> DFSTIPIDYVKAKDPNTIDFCLSYLELYHTTKAVKACTPFSFILGSDAGMQRATETTESLYWGKVILDINPNLSPLVNTTIVLEIESMLSSNSINRSENKRITRYIEKENFVNESSERFEFFKSMELSHLSTAYDVYVTFIGFKIDL

In this study, we report a detailed characterization of ΦCjT23, an icosahedral temperate ssDNA phage with an inner lipid membrane, isolated earlier from a strain of Flavobacterium (previously Cytophaga). The virion structure determined by cryogenic electron microscopy reveals similarities to members of the viral kingdom Bamfordvirae that currently consists solely of dsDNA viruses with a major capsid protein composed of two upright β-sandwiches. The minimalistic structure of ΦCjT23 suggests that this phage serves as a model for the last common ancestor between ssDNA and dsDNA viruses in the Bamfordvirae. Both ΦCjT23 and the related phage FLiP infect Flavobacterium species found in several environments, suggesting that these types of viruses have a global distribution and a shared evolutionary origin.

Earlier, we reported a phylogenetic connection between phage PM2 and the ssDNA phage FLiP (Finnlakevirus FLiP, Finnlakeviridae), which infects flavobacteria. Structurally, however, the two share the same capsid organization, characterized by the triangulation (T) number pseudo T = 21 dextro. Following the approach applied to the MCPs, we calculated a localized reconstruction of the internal part of ΦCjT23 spike (penton domain), in addition to the FLiP penton base from our previously published data. The resolutions of the localized reconstructions for ΦCjT23 and FLiP were 3.4 and 4.0 Å, respectively. This was sufficient to build the corresponding atomic models de novo. As expected, the structure of the FLiP penton revealed a pentamer formed by five copies of protein P12 (encoded by orf12) with the canonical β-sandwich fold, similar to penton base proteins of PM2 and PRD1. This confirmed that the FLiP spike is formed by a separate protein forming a pentamer sitting atop the capsid integral penton base.> GGSGQTQPLKSVFSIDAGRKYFSVEQLEELVAKASQNGYTDVQLILGNDGLRFILD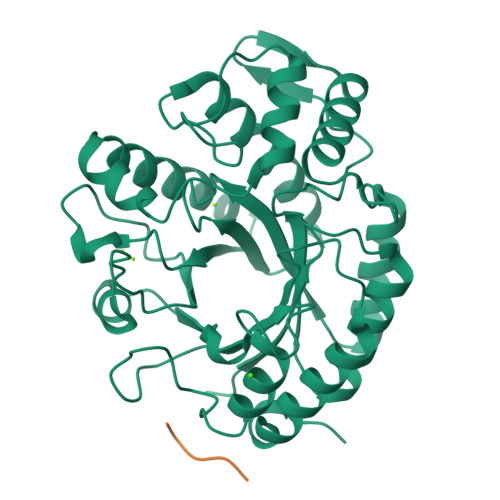DMSVNVNGKKYNHNRVSKAIQRGNNAYYNDPNGNALTQKEMDRLLAFAKARNINIIPVINSPGHMDALLVAMEKLAIKNPAFDGSKRTVDLGNQKAVNFTKAIISKYVAYFSAHSEIFNFGGDEYANDVDTGGWAKLQSSGRYKDFVAYANDLAKIIKDAGMQPMSFNDGIYYNSDDSFGTFDPEIIISYWTAGWSGYDVAKPEYFVQKGHKIFNTNDAWYWVAGNVDSGIYQYDDALANMSKKAFTDVPAGSPNLPIIGSIQCVWYDDPRRDYDFERIYTLMDTFSENYREYMVVKNH;> GAGAA> MLMPKKERKVEGDEVIRVPLPEGNQLFGVVEQALGAGWMDVRCEDGKIRRCRIPGKLRRRVWIRVGDLVIVQPWP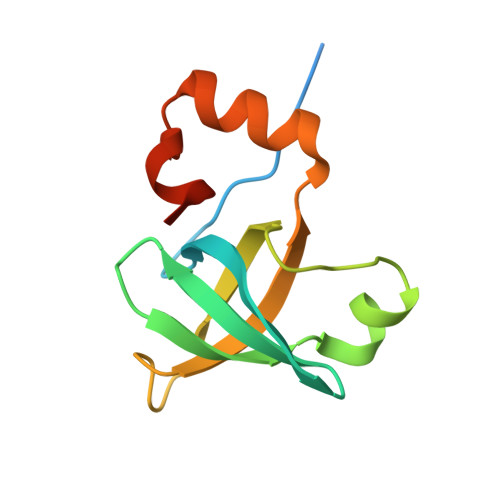VQSDKRGDIVYRYTQTQVDWLLRKGKITQEFLTGGSLLVE>MASATLPRFDLMGWDKKDIADPYPVYRRYREAAPVHRTASGPGKPDTYYVFTYDDVVRVLSNRRLGRNARVASGDTDTAPVPIPTEHRALRTVVENWLVFLDPPHHTELRSLLTTEFSPSIVTGLRPRIA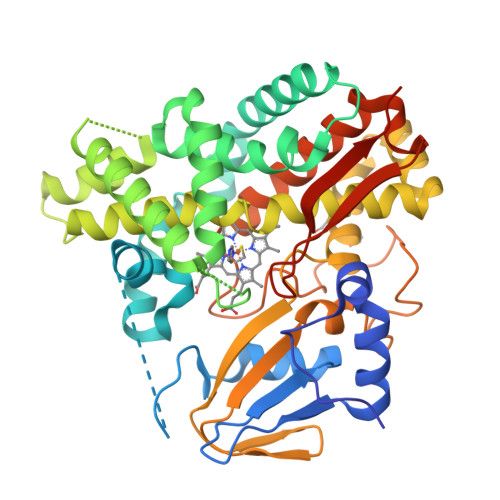ELASALLDRLRAQRRPDLVEGFAAPLPILVISALLGIPEEDHTWLRANAVALQEASTTRARDGRGYARAEAASQEFTRYFRREVDRRGGDDRDDLLTLLVRARDTGSPLSVDGIVGTCVHLLTAGHETTTNFLAKAVLTLRAHRDVLDELRTTPESTPAAVEELMRYDPPVQAVTRWAYEDIRLGDHDIPRGSRVVALLGSANRDPARFPDPDVLDVHRAAERQVGFGLGIHYCLGATLARAEAEIGLRALLDGIPALGRGAHEVEYADDMVFHGPTRLLLDLPDAALEHHHHHH[4x]>[2x]GSMGKPFFTRNPSELKGKFIHTKLRKSSRGFGFTVVGGDEPDEFLQIKSLVLDGPAALDGKMETGDVIVSVNDTCVLGHTHAQVVKIFQSIPIGASVDLELCRGYPLGSSAYGSVKAYTNFDAERDALNIETAIKT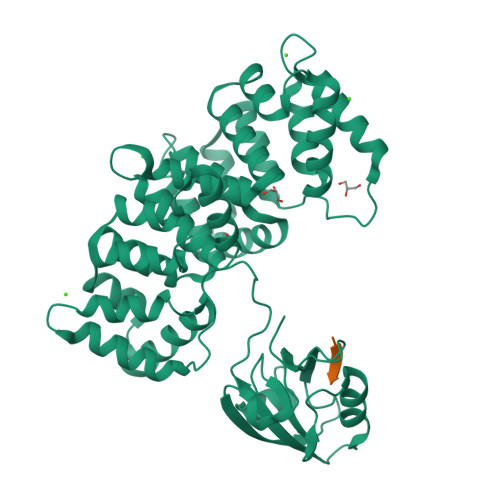KGVDEVTIVNILTNRSNEQRQDIAFAYQRRTKKELASALKSALSGHLETVILGLLKTPAQYDASELKASMKGLGTDEDSLIEIICSRTNQELQEINRVYKEMYKTDLEKDIISDTSGDFRKLMVALAKGRRAEDGSVIDYELIDQDARDLYDAGVKRKGTDVPKWISIMTERSVPHLQKVFDRYKSYSPYDMLESIRKEVKGDLENAFLNLVQCIQNKPLYFADRLYDSMKGKGTRDKVLIRIMVSRSEVDMLKIRSEFKRKYGKSLYYYIQQDTKGDYQKALLYLCGGDD;> GSQDLQLVKGAMAATYSALNSSKPTPQLKPIESSILAQRRVRKLPSTTL> TSAVLLDHCHFSQVIFNSVEKFYIPGGDVTCHYTFTQHFIPRRKDWIGIFRVGWKTTREYYTFMWVTLPIDLNNKSAKQQEVQF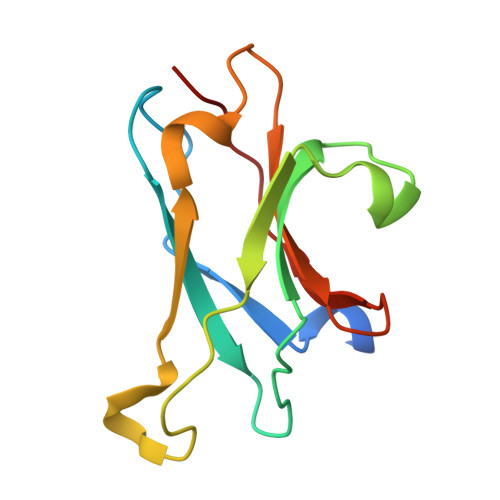KAYYLPKDDEYYQFCYVDEDGVVRGASIPFQFR> AANAPGGSNVVNETPAQTVEVRAAPDALAFAQTSLSLPANTVVRLDFVNQNNLGVQHNWVLVNGGDDVAAAVNTAAQNNA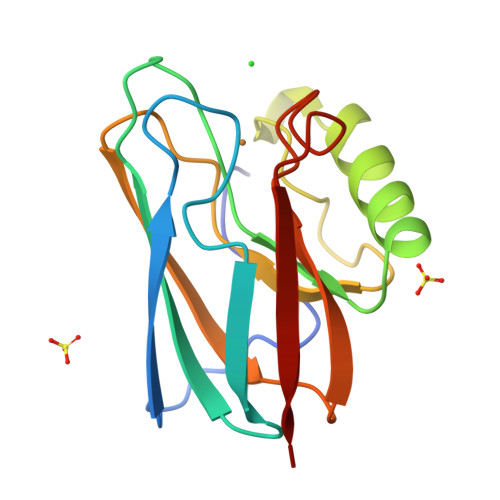DALFVPPPDTPNALAWTAMLNAGESGSVTFRTPAPGTYLYICTFPGHYLAGMKGTLTVTP>[4x]MGSDK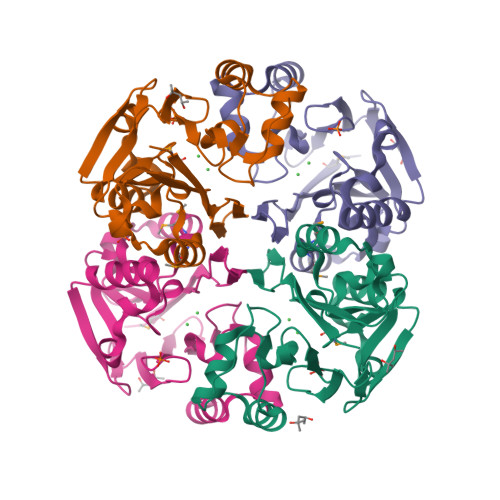IHHHHHHMELKILVTGGNVFVPGRLNAHFSTVVYLEHKDRRIIIDPGNLSSMDELEEKFSELGISPDDITDVLFTHVHLDHIFNSVLFENATFYVHEVYKTKNYLSFGTIVGRIYSKVISSWKNVVLLKGEESLFDEKVKVFHTPWHAREHLSFLLDTENAGRVLITGDITPNRLSYYDIIKGYGSVQVKNFLDRVGRIDLLVFPHDAPLKPEVKK> SRRARIERRTRESDIVIELDLDGTGQVAVDTGVPFYDHMLTALGSHASFDLTVRATGDVEIEAHHTIEDTAIALGTALGQALGDKRGIRRFGDAFIPMDETLAHAAVDLSGRPYCVHTGEPDHLQHTTIAGSSVPYHTVINRH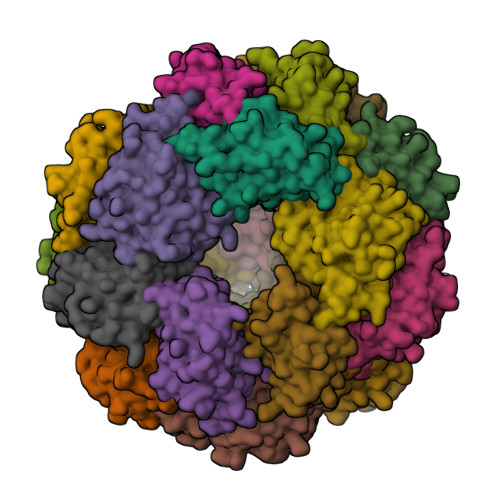VFESLAANARIALHVRVLYGRDPHHITEAQYKAVARALRQAVEPDPRV> MKHIKILNGSTLKDSL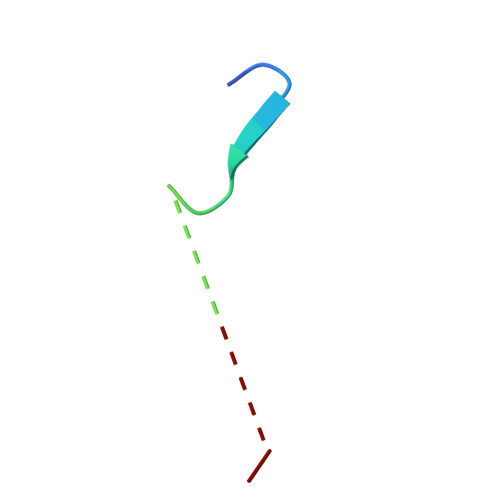KKGGC> MLQYRIIVDGRVQGVGFRYFVQ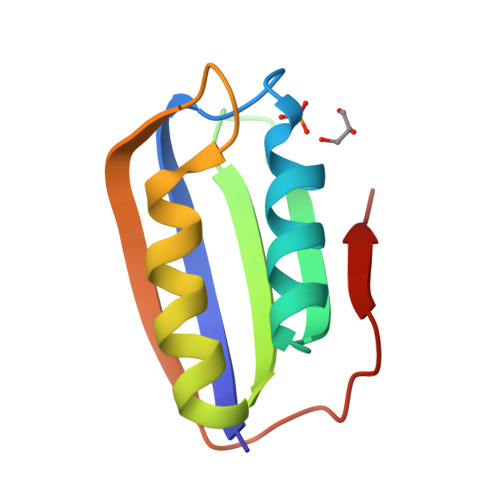MEADKRKLAGWVKNRDDGRVEILAEGPENALQSFVEAVKNGSPFSKVTDISVTESRSLEGHHRFSIVYS>[2x]LSKNVVAVNEELTAEEWKRRYEKEKEKNAR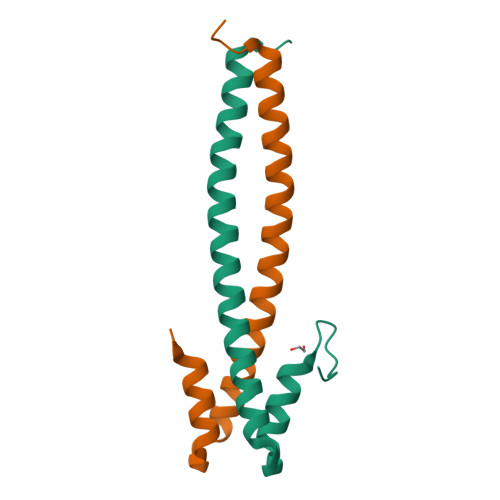LKGKVEDLEKERDFYFGKLRNIELICQENEGENDPVLQRIVDILYATDEGFVIPD> MSWRHIRAEGLDSS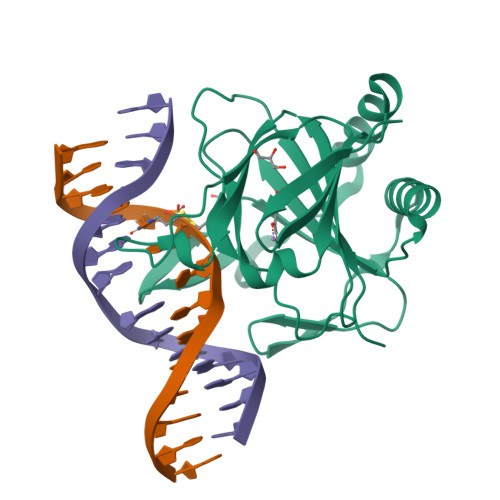YTVLFGKAEADEIFQELEKEVEYFTGALARVQVFGKWHSVPRKQATYGDAGLTYTFSGLTLSPKPWIPVLERIRDHVSGVTGQTFNFVLINRYKDGSDHICEHRDDERELAPGSPIASVSFGASRDFVFRHKDSRGKSPSRRVAVVRLPLAHGSLLMMNHPTNTHWYHSLPVRKKVLAPRVNLTFRKILL> MADFLNFPRQMLPFSKKTKQWRKDCLLWANQKTFFNYSLVRKSVIHKKINYDLLNGRLHMSDLELVLNPDGIKAAYIPDRLQHYPIMNSKLNVLRGEESKRVFDFKVVVTNPNAISEIEDNKKNELLQRLQEMITDTSISEDEYNIKLEKLNDYYTYEWQDIREVRANELLNHYIKEYDIPLIFNNGFMDAMTCGEEIYQCDIVGGEPVIERVNPLKIRIFKSGYSNKVEDADMIILEDYWSPGRVIDTYYDVLSPKDIKYIETMPDYIGQGAVDQMDNIDERYGFVNQNMIGDEITVRDGTYFFDPANLFTEGIANSLLPYDLAGNLRVLRLYWKSKRKILKVKSYDPETGEEEWNFYPENYVVNKEAGEEVQSFWVNEAWEGTMIGNEIFVNMRPRLIQYNRLNNPSRCHFGIVGSIYNLNDSRPFSLVDMMKPYNYLYDAIHDRLNKAIASNWGSILELDLSKVPKGWDVGKWMYYARVNHIAVIDSFKEGTIGASTGKLAGALNNAGKGMIETNIGNYIQQQINLLEFIKMEMADVAGISKQREGQISQRETVGGVERATLQSSHITEWLFTIHDDVKKRALECFLETAKVALKGRNKKFQYILSDTSTRVMEIDGDEFAEADYGLVVDNSNGTQELQQKLDTLAQAALQTQTLSFSTITKLYTSSSLAEKQRLIEKDEKQIRERQAQAQKEQLEAQQQIAAMQQQQKEAELLQKEEANIRDNQTKIIIAQIQSEGGPDEEDGIMIDDYSPEAKANLAEKIREFDEKLKLDKDKLKLDKKKAETDASIKRQALRKKSSTTNK;> MVNNINWVKLPVILDRLLRHPLLTDLNLETAIQYTLDFISAMGLPNVYVDKIETIDIKEYRGELPCDLISINQVRLHKNGIALRAMTDNFNAYPTHDHKEGDWYERGEPSFKTQGRVIFTSIKHEKVDISYKAIMLDDEGLPLIPDNPIFLKTLELYIKKEWFTILFDMGKISPAVLNNTQQEYAFKAGQCNNEFVIPSVSEMEAITNMWNQLIPRVTEFRRGFKNLGDKEYIRVH;> MTYNELIYMVLDELKLSSDDSYYTPDHVIFLLVKYRSFLLKQRYSDIKKQIPDSDYQSICLDLIEVPAISGEPCEGSSYLRSKNKVPTTMMIGNPRVYPMDFYQGEITYISRDRMRYVGYNKFLRNIIYCSKAPDGYLYFKSWNPQFLHLEKVSFNAIFEDAKEASEMACPEENGTICKLEDKEFPIEDALVPPLIELVVKELRGPEYSPKDEDNNAKDDLPDAR;>[2x]MAKKKIKRRGKMPPNIFDTGGQSWGQQSSGQFSNAFKGENLGNSIGSIGGAVGGIAQAGISNAQIADTSGIEAQNKAQKNMVVGASSNDDLMSEWGSWNKVKDDYSWKDVRGGSTGQRVTNTIGAAGQGAAAGASVGGPIGAIVGGVVGLGSAIGGWLGGNRKAKRKAKKLNKEAKEANERALTSFETRADNIDTQNDFNMLANFSAYGGPLEFGSGAIGYEFDNRYLNNQEMSAVAKQRLTSLPNSFQALPEMNTYNAFAEGGGLSREKNYGSKKKPYPSVPSGDFAGPHRSYPIPTKADARDALRLAGLHGNESVRRKVLAKYPSLKAFGGSLFDSVVGNNFNQSFTQGIQGMFQQEPEQTVQAANIAKDGGDIKIKEKNKGKFTAYCGGKVTEACIRKGKNSSNPTTRKRATFAQNARNWNAFGGWLNTQGGDFTNGVTFINEGGSHEENPYQGIQIGVDPEGAPNLVEQGEVVYDDYVFSDRMEIPDDIRKEYKLRGKTFAKAAKSAQRESEERPNDPLSTKGLQAAMERIATAQEEARQRKEAHREGNEYPSMFAYGGDTNPYGLALEDPMSVEELEALMVQSGETGEIAPEGNNGNRQTWTRYAPIIGSGLASLSDLFSKPDYDSADLISGVDLGAEAVGYAPIGNYLSYRPLDRDFYINKMNQQAAATRRGLMNTSGGNRLNAQAGILAADYNYGQNMGNLARQAEEYNQQLRERVEAFNRGTNMFNTETGLKASMFNAESRNAAKRARLGQATTVAQLRQGIKDQDAARRSANITNFLQGLGDMGWENEQANWLDTLAKSGVLKMNTKGEYTGGTKKAKGGKVRTKKKKGLTYG

Virus ΦcrAss001 (Kehishuvirus primarius) was the first representative of this order to be isolated in pure culture from human faecal samples. Here, we present the characterization of ΦcrAss001 using cryo-electron microscopy (cryo-EM), enabling de novo structure building and elucidation of functions for around 1,440 protein subunits constituting the virion, leading to the identification of a novel ‘crass fold’ in the distal part of the tail. The virion possesses a short non-contractile tail extending approximately 44 nm from an icosahedral capsid. The extended tail barrel formed by widely conserved paralogous ring proteins has a high capacity for storage of cargo proteins alongside the capsid cargo zone, ensuring that the proteins required for the initial stages of crassvirus infection are carried inside virions and delivered to the host cell.

The majority of the portal protein oligomer exhibits 12-fold symmetry and the localized reconstruction imposing C12 symmetry enabled structure determination at 3.09 Å resolution. The majority of the portal protein residues, except for some flexible loop segments (33–35, 68–71, 269–324 and 550–563), could be confidently modelled. At the top of the portal protein, an extended α-helical barrel (C-terminal residues 672–739) extends around 80 Å towards the core of the capsid. This extended feature has an internal van der Waals diameter of around 45 Å at the base of the crown and around 25 Å at its exposed end. The main body of the portal protein beneath the Crown domain is made up of the stem domain, composed of α-helices defining its central tunnel, and the wing domain. Tunnel loops, which are not defined in maps owing to their apparent flexibility, connect the inner stem helix (residues 519–541) with a 34-residue-long kinked helix that is part of the wing. These tunnel loops (residues 550–563) are likely to form a narrow constriction in the portal tunnel, as observed in portal proteins of other viruses. At the surface of the portal wing, there is clear density corresponding to residues 425–552 of the gp45 cargo protein C1. Twelve such segments of gp45 interdigitate with wing loops (SH3-like domains) of the portal, residues 337–380.>[2x]QAQITGRPEWIWLALGTALM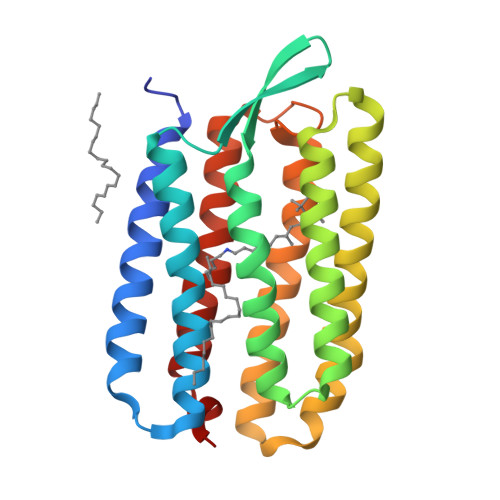GLGTLYFLVKGMGVSDPDAKKFYAITTLVPAIAFTMYLSMLLGYGLTMVPFGGEQNPIYWARYADWLFTTPLLLLDLALLVDADQGTILALVGADGIMIGTGLVGALTKVYSYRFVWWAISTAAMLYILYVLFFGFTSKAESMRPEVASTFKVLRNVTVVLWSAYPVVWLIGSEGAGIVPLNIETLLFMVLDVSAKVGFGLILLRSRAIFG(2~{R})-2-(4-phenylphenoxy)propanoic acid | C15 H14 O3 | 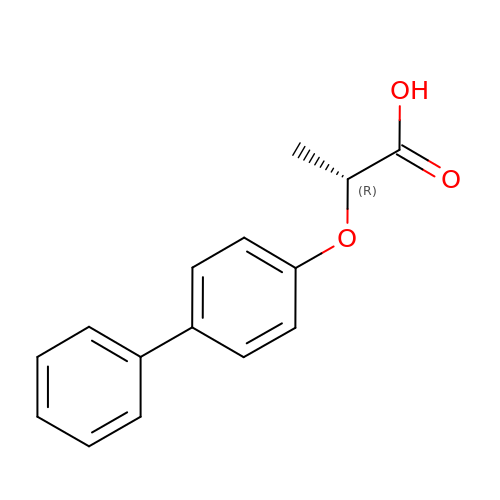FUPGQEMJIGUBGO-LLVKDONJSA-N>MAHHHHHHMTSVGLIWAQSTSGVIGRDGGIPWRLPEDLAHFKRLTMGHTVVMGRRTWDSLPAAHRPLPGRRNVVVTRQTGLVAHGAQVVGSLEQALSPAEPDAATWVIGGAQIYALALPLANRCEVTEVDVDLPPEDEDALAPVLDQTWAGT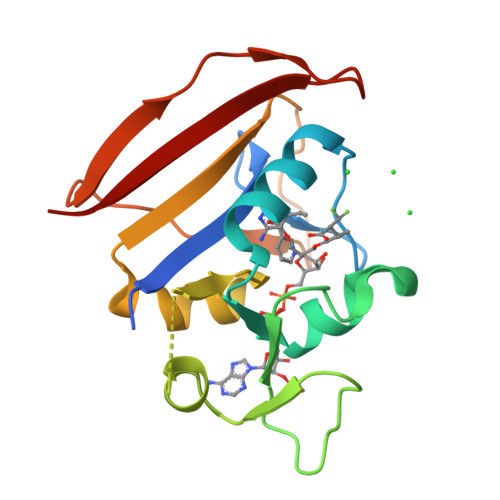SGEWLVSRSGLRYRMHSYRRL[2x]> GGSGGSGGMGEQPIFTTRAHVFQIDPSTKKNWVPASKQAVTVSYFYDVTRNSYRIISVDGAKVIINSTITPNMTFTKTSQKFGQWADSRANTVFGL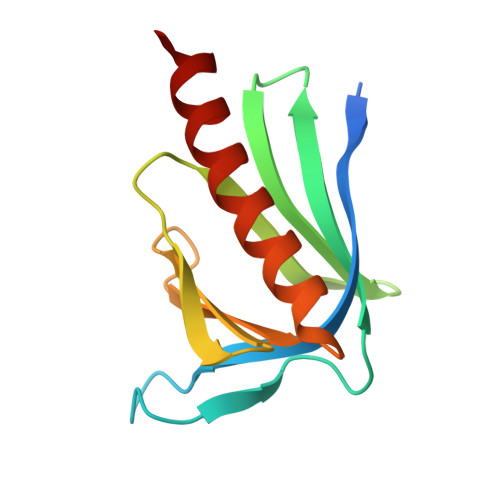GFSSELQLTKFAEKFQEVREAARLARD>[2x]MGSDKIHHHHHHENLYFQGHMTTVSTNDFDQQHLWHPYASLPPTYPNIVIDRAEGIYIVTEDGTRLIDGMSSWWASVHGYNHPKLNAAMIEQLGKMAHVMFGGLTHQPAIDLGKKLLSIVPAGLDAIFYADSGSIAVEVALKMALQYQIAAKRPSKCQFASTHSGYYGDTWHAMSVCDPINGMHSLYGKQLPMQHFVAAPPMG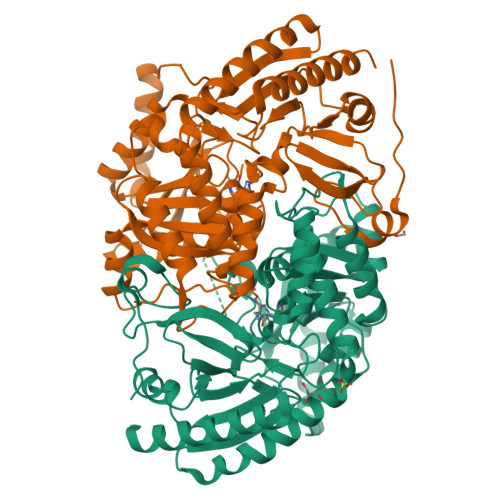FERDLTQSEREALTEFFVKNSDKLAGFIIEPIIQGAGGMRFYSPQYLQLLRKLCDEYDVLLIADEIATGFGRSGKLFACEHAAISPDIMTIGKALTGGYMTFAATLSTREIADTISQSDYPALMHGPTFMGNPLACAVACASIDLIVSYDIEARTENMQAIMNEQLAPAVSLEGVKEVRCLGAVAVIELNEAVDMPIFQTLLINNGIWVRPFGKLVYIMPPYVITDDELTTLCQALLKVVSSYLTRKD5'-O-(L-phenylalanylsulfamoyl)adenosine 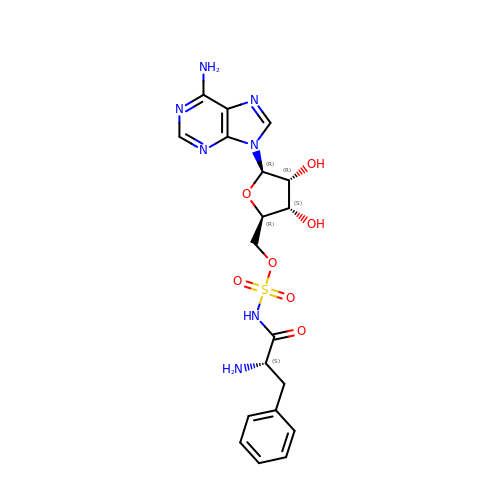| C19 H23 N7 O7 S | QGOJGCAOMCBQFJ-QTOWJTHWSA-N> MEKNFVISDPRLPDNPIIFASDSFLELTEYSREEILGRNCRFLQGPETDQATVQKIRDAIRDQREITVQLINYTKSGKKFW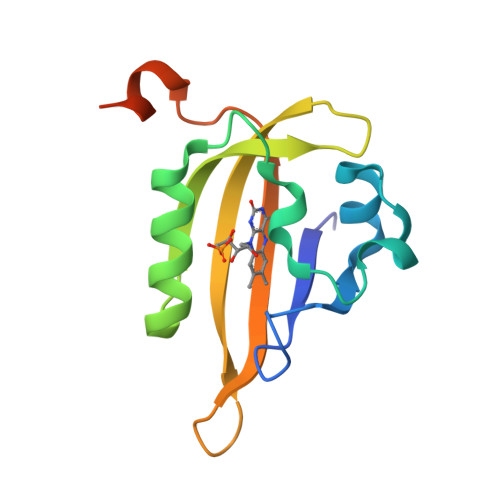NLFHLQPMRDQKGELQYFIGVQLDGEFIPNPLLGLDSTRTGHHHHHH> MTDQNLPVTVAGLGPMGSALAAALLDRGHDVTVWNRSPGKAAPLVA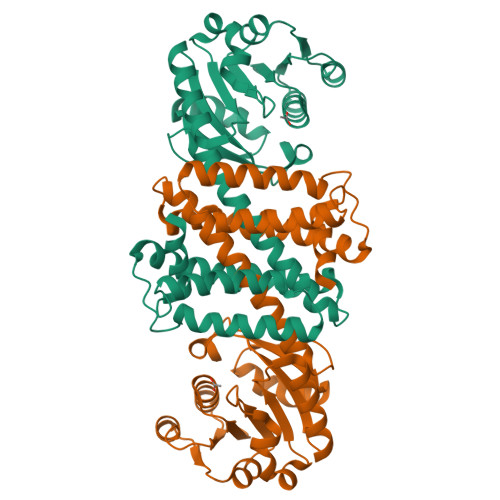KGARQADDIVDAVSASRLLVVCLADYDALYSALGPAREALRGRVVVNLNSGTPKEANEALRWAERHGTGYLDGAIMVPPAMVGHPGSVFLYSGSAEVFEEYKETLAGLGDPVHLGTEAGLAVLYNTALLSMMYSSMNGFLHAAALVGSAGVPAAEFTKLAVDWFLPAVIGQIIKAEAPTIDEGVYPGDAGSLEMNVTTLKHIIGTSQEQGVDTEIPVRNKELLDRAVAAGFGESSYYSVIELWR> MDPLRAQQLAAELEVEMMADMYNRMTSACHRKCVPPHYKEAELSKGESVCLDRCVSKYLDI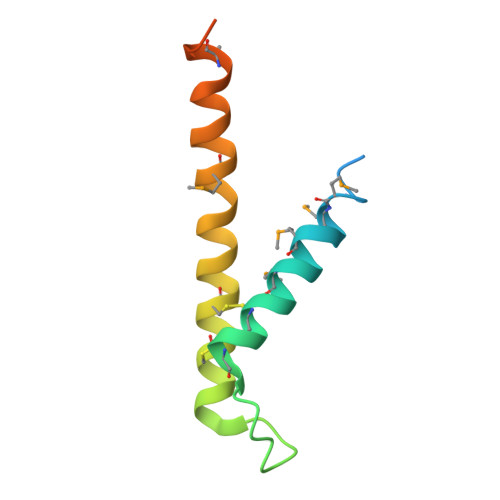HERMGKKLTELSMQDEELMKRVQQSSGPA> S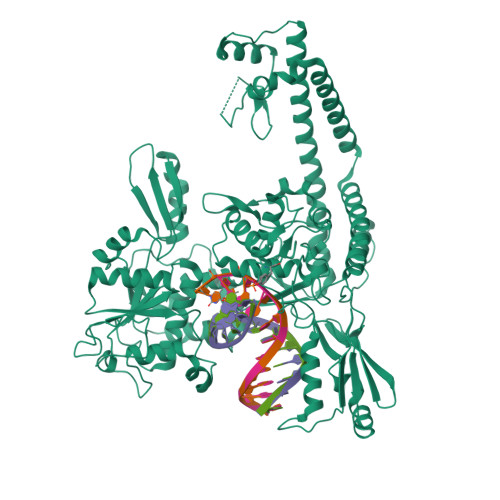RITNYPKLEDANKAGTKEGYKCTLVLTEGDSALSLAVAGLAVVGRDYYGCYPLRGKMLNVREASADQILKNAEIQAIKKIMGLQHRKKYEDTKSLRYGHLMIMTDQDHDGSHIKGLIINFLESSFPGLLDIQGFLLEFITPIIKVSITKPTKNTIAFYNMPDYEKWREEESHKFTWKQKYYKGLGTSLAQEVREYFSNLDRHLKIFHSLQGNDKDYIDLAFSKKKADDRKEWLRQYEPGTVLDPTLKEIPISDFINKELILFSLADNIRSIPNVLDGFKPGQRKVLYGCFKKNLKSELKVAQLAPYVSECTAYHHGEQSLAQTIIGLAQNFVGSNNIYLLLPNGAFGTRATGGKDAAAARYIYTELNKLTRKIFHPADDPLYKYIQEDEKTVEPEWYLPILPMILVNGAEGIGTGWSTYIPPFNPLEIIKNIRHLMNDEELEQMHPWFRGWTGTIEEIEPLRYRMYGRIEQIGDNVLEITELPARTWTSTIKEYLLLGLSGNDKIKPWIKDMEEQHDDNIKFIITLSPEEMAKTRKIGFYERFKLISPISLMNMVAFDPHGKIKKYNSVNEILSEFYYVRLEYYQKRKDHMSERLQWEVEKYSFQVKFIKMIIEKELTVTNKPRNAIIQELENLGFPRFNKEGKPYYGSPNDEIAEQINDVKGATSDEEDEESSHEDTENVINGPEELYGTYEYLLGMRIWSLTKERYQKLLKQKQEKETELENLLKLSAKDIWNTDLKAFEVGYQEFLQRDAEAR> GSAHASVIKPEMKIKLRMEGAVNGHKFVIEGEGIGKPYEGTQTLDLTVEEGAPLPFSYDILTPAFQYGNRAFTKYPEDIPDYFKQAFPEGYSWERSMTYEDQGICIATSDITMEGDCFFYEIRFDGTNFPPNGPVMQKKTLKWKSPTGKMYVEDGVLKGDVEMALLLEGGGHYR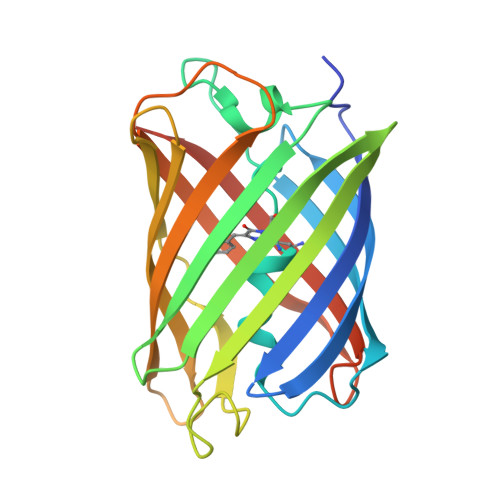CDFKTTYKAKKDVRLPDAHEVDHRIEILSHDKDYNKVRLYEHAEARYSGGGSGGGAS> MAFTRAFLSKSTVEFGQDNFLTCPLGILFTLGILLGSGGAQGKTGHQIGKAIRLKSTSSSWNPFGAQEEMKSLYKELNDSLGSEKTFIDDKEEKVVRISTGLFVQRTHEIETSFNESIKNDFKGELIPVNFLNRTSATLSINRWVDQQSNGLLEKFFMDDIPDDTGMILVNVFYFRDFWESPFEPHYTKIENFDISPNRQIKVPMMMKEEVLHYGKFENQGFEIVSKPLNNTRFTFVVVLPLEKWSLTGAMELLNGNKILSEYIKKLKETTVSLRLPKFTLKNTLDLVQTLKSMGIVDLFNPVAANLSGITHDHQLYVDKFMQTNILKLNESGIEATTVTSPIFVPISAVLPDIDFNVNHPFICFIYDQQLTMPIIAAKVIEPIISSA

Serpins are proteins distributed among all kingdoms of life that act mostly as Serine protease inhibitors, but also as inhibitors of other classes of proteases, although some that lack inhibitory activity can serve as chaperones or storage proteins. Serpins from parasites are interesting immunodiagnostic targets, due to their presence at the parasite-host interface, where they are crucial for the adaptation and survival of the parasite to the host environment by modulating inflammatory response. Among these, SmSPI is able to weakly inhibit chymotrypsin and is expressed mostly in the parasite’s head gland, confirming its localization in the parasite-host interface, thus its potential as a diagnostic target.

In this context, we present the 3.22 Å resolution crystal structure of the S. mansoni circulating antigen SmSPI together with flanking immune sera recognition tests using sera from affected patients. One protein molecule was found in the crystal asymmetric unit, with an estimated solvent content of 67 % (Matthew’s coefficient = 3.78 Å3/Da). The SmSPI structure presents the fold and topology of a canonical Serpin composed of 3 β-sheets (named βA, βB, βC, assigned according to the conventional Serpin nomenclature) and 10 α-helices. Electron density was well defined for the main chain atoms except for some flexible, loop regions. The major region with no electron density is the Reactive Centre Loop (RCL; residues 357 to 368), which is highly flexible and solvent exposed; its function is indeed to act as a bait for the target protease to exert the Serpin inhibitory activity. Other poor electron density regions were for several solvent exposed loops (AA 35–36, 107–108, 262–263), in accordance with other deposited Serpin structures. Three SmSPI epitopes were identified: Ep1: 123-VQRTHEIETSFNE-135; Ep2: 175-FMDDIPDDTG-185; Ep3: 320-NPVAANLSGITHDHQLYVD-338. All three identified epitopes are clustered together in the same region of the protein. SmSPI showed to be able to bind human IgG in sera from people affected by Schistosomiasis, while the response of the protein to healthy serum resulted to be significantly lower (p < 0.001).> MTVARPSVPAALPLLGELPRLLLLVLLCLPAVWQDCGLPPDVPNAQPALEGRTSFPEDTVITYKCEESFVKIPGEKDSVICLKGSQWSDIEEFCNRSCEVPTRLNSASLKQPYITQNYFPVGTVVEYECRPGYRREPSLSPKLTCLQNLKWSTAVEFCKKKSCPNPGEIRNGQIDVPGGILFGATISFSCNTGYKLFGSTSSFCLISGSSVQWSDPLPECREIYCPAPPQIDNGIIQGERDHYGYRQSVTYACNKGFTMIGEHSIYCTVNNDEGEWSGPPPECRGKSLTSKVPPTVQKPTTVNVPTTEVSPTSQKTTTKTTTPNAQATRSTPVSRTTKHFHETTPNKGSGTTSGTTRLLSGHTCFTLT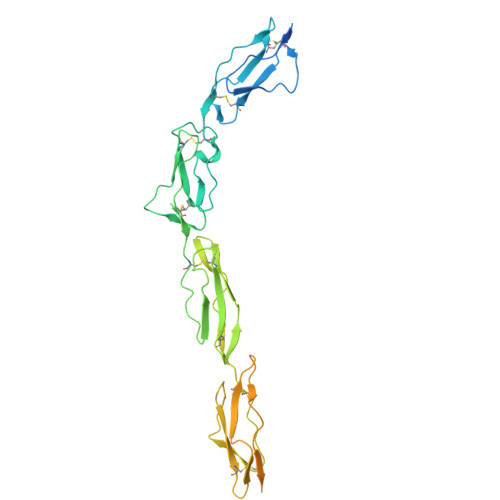GLLGTLVTMGLLT N-[(2Z,5R,7R,8S,9S,10R)-8,9,10-trihydroxy-7-(hydroxymethyl)-4-oxo-6-oxa-1-thia-3-azaspiro[4.5]dec-2-ylidene]naphthalene-2-carboxamide | C19 H18 N2 O7 S 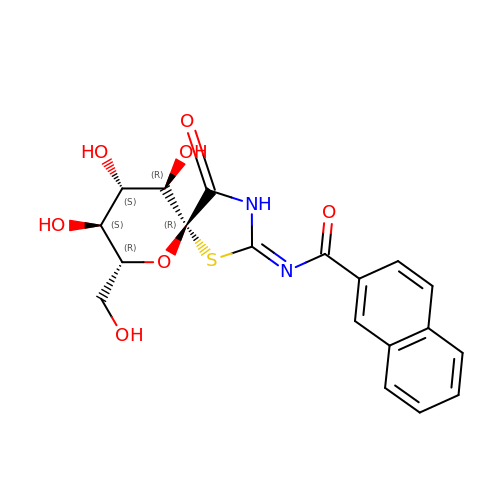| YJXSIZXIPBKFHB-ULPMNANESA-N Ursolic acid  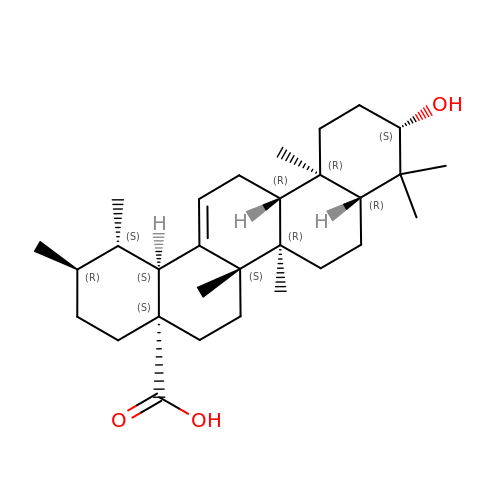| C30 H48 O3 | WCGUUGGRBIKTOS-GPOJBZKASA-N> MEPPVQVAVIGSGGAAMAAALKAVEQGAQVTLIERGTIGGTAVNVGAVPSKIMIRAAHIAHLRRESPFDGGIAATVPTIDRSKLLAQQQARVDELRHAKYEGILGGNPAITVVHGEARFKDDQSLTVRLNEGGERVVMFDRCLVATGASPAVPPIPGLKESPYWTSTEALASDTIPERLAVIGSSVVALELAQAFARLGSKVTVLARNTLFFREDPAIGEAVTAAFRAEGIEVLEHTQASQVAHMDGEFVLTTTHGELRADKLLVATGRTPNTRSLALDAAGVTVNAQGAIVIDQGMRTSNPNIYAAGDCTDQPQFVYVAAAAGTRAAINMTGGDAALDLTAMPAVVFTDPQVATVGYSEAEAHHDGIETDSRTLTLDNVPRALANFDTRGFIKLVIEEGSHRLIGVQAVAPEAGELIQTAALAIRNRMTVQELADQLFPYLT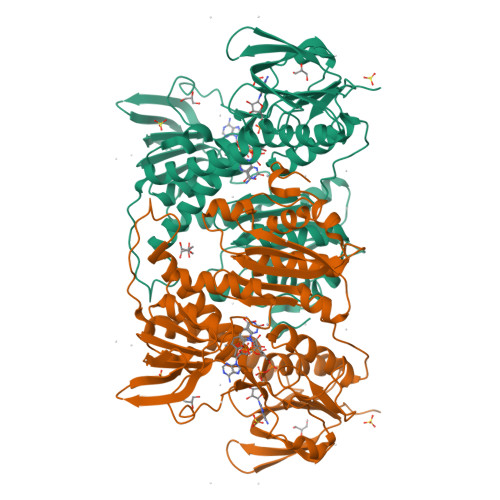MVEGLKLAAQTFNKDVKQLSCCAG> ATSWLLDGHLRAYTDDLARRLRGEPNAHLLHFADSQVVTMLSSADPDQQARAQRLLAGDDIPPIVFLPINQPNAHWSLLVVDRRNKDAVAAYHYDSMAQKDPQQRYLADMAAYHLGLDYQQTHEMPIAIQSDGYSAGDHVLTGIEVLAHRVLDGTFDYAGGRD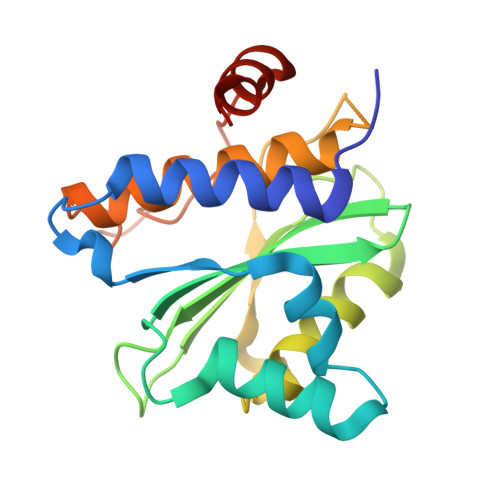LTDIEPDRGLIRDRLAQAEQAPA> GSPGIRLGSSEDNFARFVCKNNGVLFENQLLQIGLKSEFRQNLGRMFIFYGNKTSTQFLNFTPTLICADDLQTNLNLQTKPVDPTV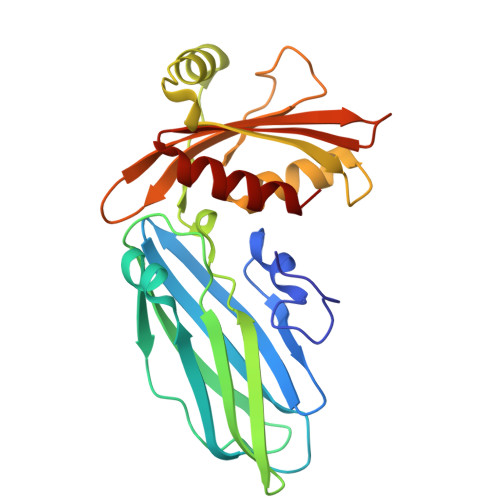DGGAQVQQVVNIECISDFTEAPVLNIQFRYGGTFQNVSVKLPITLNKFFQPTEMASQDFFQRWKQLSNPQQEVQNIFKAKHPMDTEITKAKIIGFGSALLEEVDPNPANFVGAGIIHTKTTQIGCLLRLEPNLQAQMYRLTLRTSKDTVSQRLCELLSEQF Described herein are the 3D structures of two stereoselective pterocarpan-forming DPs from pea and licorice, which preferentially produce either (+)- or (–)-medicarpin, depending on the substrate. We describe that pterocarpan synthases, containing dirigent-like domains, initially engender mono-QM formation from their chiral substrates, this being followed by intramolecular cyclization (C–O bond formation) to afford entry into the pterocarpan natural product (phytoalexin) class. GePTS1 and PsPTS1, in solution, exist mainly as trimers (∼68.0 kDa), with (because of association/aggregation) a small amount of higher-molecular weight entities also being evident (roughly corresponding to 410–500 kDa). The entrance to the putative active site of the GePTS1 and PsPTS1 monomers is located at the end of the barrel opposite the N and C termini.

The P. sativum “Cam_eor” Unigene set was searched using GePTS1 as query, which resulted in a gene (PsCam039127) being selected as possibly encoding a medicarpin-forming DP. Trivially named PsPTS1, it has ∼92%/85% sequence similarity/identity to GePTS1 at the amino acid level. In our hands, PsPTS1 displayed much lower (∼7-fold) catalytic turnover (kcat/Km) relative to GePTS1, this in part being due to the ∼6-fold increase in Km. The pea medicarpin-forming DP, PsPTS1, structure was solved by single-wavelength anomalous diffraction methods using the signal from intrinsic sulfur atoms (sulfur-SAD (single anomalous diffraction)) in the 11 methionine residues (excluding the N-terminal methionine). Its structure was refined against 1.5 Å resolution native data to a final Rfree of 0.1907. It consists of a single monomer in the asymmetric unit, residues Phe35–Tyr187, plus two residues at the C terminus (Lys188 and Gly189) from the linker for the C-terminal His tag. The extended N terminus observed in some of the GePTS1 monomers is not resolved in the PsPTS1 structure. A trimeric complex is formed by the crystallographic 3-fold axis parallel to the body diagonal of the cubic unit cell, this being in agreement with the GPC. PsPTS1 also has an eight-stranded β-barrel structure, comprised of two curved β-sheets with the same topology as GePTS1 (sheet I: β1′, β2, β3, β4, β5, and β6′; sheet II: β6, β7, β8, and β1). The PsPTS1 and GePTS1 monomer structures are thus very similar, with RMSDs between 0.47 and 0.75 Å for the superposition of the PsPTS1 monomer on the six independent GePTS1 monomers.

> MTKYYQSLSPTMLGFQEEKFTHLHFYFHDIVTGPKPSMVFVAEPNGKVENALPFGTVVAMDDPLTAGPERDSKLVGKAQGIYTSISQEEMGLMMVMTMAFSDGEFNGSTLSILGRNMIMSETIREMAIVGGTGAFRFVRGYAQAKFFSVDFTTGDATVEYDIFVFHYKGELNSKLEGKPIPNPLLGLDSTRTGHHHHHH> MDSTSTIANKIEEYLGAKSDDSKIDELLKADPSEVEYYRSGGDGDYLKNNICKITVNHSDSGKYDPCEKKLPPYDDNDQWKCQQNSSDGSGKPENICVPPRRERLCTYNLENLKFDKIRDNNAFLADVLLTARNEGEKIVQNHPDTNSSNVCNALERSFADLADIIRGTDQWKGTNSNLEKNLKQMFAKIRENDKVLQDKYPKDQKYTKLREAWWNANRQKVWEVITCGARSNDLLIKRGWRTSGKSDRKKNFELCRKCGHYEKEVPTKLDYVPQFLRWLTEWIEDFYREKQNLIDDMERHREECTREDHKSKEGTSYCSTCKDKCKKYCECVKKWKTEWENQENKYKDLYEQNKNKTSQKNTSRYDDYVKDFFEKLEANYSSLENYIKGDPYFAEYATKLSFILNPSDGILQENCSDNKRGSSSNDSCDNKNQDECQKKLEKVFASLTNGYKCDKCKSGTSRSKKKWIWKKSSGNEEGLQEEYANTIGLPPRTQSLYLGNLPKLENVCEDVKDINFDTKEKFLAGCLIVSFHEGKNLKKRYPQNKNSGNKENLCKALEYSFADYGDLIKGTSIWDNEYTKDLELNLQNNFGKLFGKYIKKNNTAEQDTSYSSLDELRESWWNTNKKYIWTAMKHGAEMNITTCNADGSVTGSGSSCDDIPTIDLIPQYLRFLQEWVENFCEQRQAKVKDVITNCKSCKESGNKCKTECKTKCKDECEKYKKFIEACGTAGGGIGTAGSPWSKRWDQIYKRYSKHIEDAKRNRKAGTKNCGTSSTTNAAASTDENKCVQSDIDSFFKHLIDIGLTTPSSYLSNVLDDNICGADKAPWTTYTTYTTTEKCNKERDKSKSQSSDTLVVVNVPSPLGNTPYRYKYACQCKIPTNEETCDDRKEYMNQWSCGSARTMKRGYKNDNYELCKYNGVDVKPTTVRSNSSKLDGNDVTFFNLFEQWNKEIQYQIEQYMTNANISCIDEKEVLDSVSDEGTPKVRGGYEDGRNNNTDQGTNCKEKCKCYKLWIEKINDQWGKQKDNYNKFRSKQIYDANKGSQNKKVVSLSNFLFFSCWEEYIQKYFNGDWSKIKNIGSDTFEFLIKKCGNNSAHGEEIFSEKLKNAEKKCKENESTDTNINKSETSCDLNATNYIRGCQSKTYDGKIFPGKGGEKQWICKDTIIHGDTNGACIPPRTQNLCVGELWDKSYGGRSNIKNDTKELLKEKIKNAIHKETELLYEYHDTGTAIISKNDKKGQKGKNDPNGLPKGFCHAVQRSFIDYKNMILGTSVNIYEHIGKLQEDIKKIIEKGTPQQKDKIGGVGSSTENVNAWWKGIEREMWDAVRCAITKINKKNNNSIFNGDECGVSPPTGNDEDQSVSWFKEWGEQFCIERLRYEQNIREACTINGKNEKKCINSKSGQGDKIQGACKRKCEKYKKYISEKKQEWDKQKTKYENKYVGKSASDLLKENYPECISANFDFIFNDNIEYKTYYPYGDYSSICSCEQVKYYKYNNAEKKNNKSLCYEKDNDMTWSKKYIKKLENGRSLEGVYVPPRRQQLCLYELFPIIIKNEEGMEKAKEELLETLQIVAEREAYYLWKQYNPTGKGIDDANKKACCAIRGSFYDLEDIIKGNDLVHDEYTKYIDSKLNEIFGSSNTNDIDTKRARTDWWENETITNGTDRKTIRQLVWDAMQSGVRYAVEEKNENFPLCMGVEHIGIAKPQFIRWLEEWTNEFCEKYTKYFEDMKSKCDPPKRADTCGDNSNIECKKACANYTNWLNPKRIEWNGMSNYYNKIYRKSNKESEDGKDYSMIMAPTVIDYLNKRCHGEINGNYICCSCKNIGAYNTTSGTVNKKLQKKETECEEEKGPLDLMNEVLNKMDKKYSAHKMKCTEVYLEHVEEQLNEIDNAIKDYKL

Parasite-infected red blood cells sequester in the placenta through interaction between parasite-expressed protein VAR2CSA and the glycosaminoglycan chondroitin sulfate A (CS) abundantly present in the intervillous space. Here, we report cryo-EM structures of the VAR2CSA ectodomain at up to 3.1 Å resolution revealing an overall V-shaped architecture and a complex domain organization. Compared to other PfEMP1s, the ~310 kDa VAR2CSA ectodomain is relatively conserved among parasites. It is composed of a short N-terminal segment and six Duffy Binding-Like (DBL) domains (DBL1-DBL6) unique to VAR2CSA. Several of the DBL domains are linked by complex inter-domain (ID1-3) regions with limited or no homology among PfEMP1s yielding a DBL1-ID1-DBL2-ID2-DBL3-DBL4-ID3-DBL5-ID4-DBL6 structure.

To shed further light on how VAR2CSA binds CS, we determined the cryo-EM structure of VAR2CSA supplemented with CS purified from placental tissue (plCS). The binding of VAR2CSA to plCS in KCl buffer was measured using QCM biosensor, confirming interaction in the low nanomolar range. Comparing the complex structure to the structure solved in the absence of CS, the new data yielded a 3.1 Å resolution map overall, extending to 2.8 Å in the core region. By contrast, DBL1 and DBL5/6 were less well resolved compared to the apo structure. Thus, it is possible that the peripheral regions of the structure become flexible and potentially displaced upon plCS binding. Conversely, these data indicate that plCS does not induce any conformational changes in the core, as structures of the DBL2-ID2-DBL3-DBL4-ID3 domains were highly similar in the presence or absence of plCS. Although plCS binding affinity to VAR2CSA is in the low nanomolar range, we did not observe any additional density that could represent ligand binding in the presence of plCS. This may be due to the intrinsic heterogeneity of plCS prepared from its natural placental source. Interestingly, analysis of the surface electrostatics instead revealed a single strongly positively patch, situated in a groove that spans through the VAR2CSA core which could encompass a negatively charged CS oligosaccharide. Combined with the fact that the DBL1 domain appeared more flexible in the CS-bound cryo-EM structure, it may indicate that DBL1 acts as a cover, which protects the CS binding region from antibody recognition prior to ligand binding, and is displaced once CS is bound.>XPPGPPGPPGPPGPPGPRGPPGXGPPGPPGPPG[3x]

Collagen model peptides (CMPs) serve as tools for understanding stability and function of the collagen triple helix and have a potential for biomedical applications. At the molecular level, collagen forms a right‐handed triple helix consisting of three peptide strands, which adopt a left‐handed polyproline II (PPII) type helix conformation and are held together by interstrand hydrogen bonds. A repetitive unit of three amino acids [Xxx‐Yyy‐Gly]n with a conserved glycine (Gly, G) and all‐trans amide bonds is observed. To further study the effects determining collagen triple helix stability we investigated a series of CMPs containing synthetic diproline‐mimicking modules (ProMs), which were preorganized in a PPII‐helix‐type conformation by a functionalizable intrastrand C2 bridge.

Using common SPPS protocols, the Fmoc‐protected ProM1 and ProM2 derivatives were successfully incorporated into the [XY] position of the CMP sequence Ac‐(PPG)5‐PRG‐PPG‐[XY]G‐(PPG)3‐NH2. [a] Peptide sequence: Ac‐(PPG)5‐PRG‐PPG‐[ProM2]G‐(PPG)3‐NH2; torsion angles were averaged for the central nine amino acid triplets. KGaARegarding the overall structure, the three peptide strands adopted the typical triple‐helical conformation, and no distortion could be detected, which was underlined by comparison of key parameters and alignment with (PPG)10.21 Considering the modified positions, ProM2 units were assembled in a PPII‐type helical shape (like all the other Pro rings) and were well‐embedded into the overall structure. In combination with the fact that all ProM2 units adopted an endo,exo ring puckering (as predicted by DFT calculations), a close packing of Pro rings within the triple helix was observed. The crystal structure not only confirmed the synthetic success of introducing covalent linkages in collagen models, but also demonstrated that the triple helical structure was maintained upon this manipulation. Because of their desired endo/exo flip the proline rings of Ac‐ProM2‐OMe were positioned in space that is also occupied by proline rings in a collagen environment. In fact, this endo/exo flip could be found in a crystal structure of the ProM2‐CMP facilitating a close packing of proline residues (see below). In the case of Ac‐ProM2‐OMe, no conformer with an endo ring flip at Yyy was found in the initial conformational search (30 kJ mol−1 cutoff), demonstrating the general exo propensity of ProM2 derivatives. A pseudo‐equatorial orientation of the rigid ethylene linker relative to the Yyy ring is sterically favored and thus controls the Cγ ring flip depending on the configuration at Cδ (endo for Ac‐ProM1‐OMe, exo for Ac‐ProM2‐OMe). Regarding the reference peptide, the stability was slightly decreased for the ProM2‐CMP or maintained in the case of the H2‐ProM2‐CMP.N-ISOBUTYL-N-[4-METHOXYPHENYLSULFONYL]GLYCYL 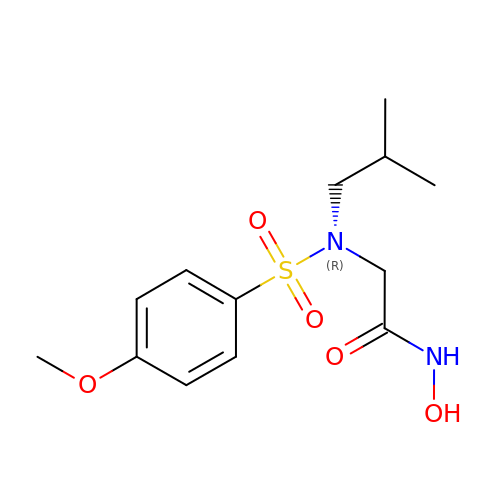HYDROXAMIC ACID | C13 H20 N2 O5 S | JIRXORZYIXSWOB-UHFFFAOYSA-N The fungal Bromodomain and Extra‐Terminal (BET) protein Bdf1 is a potential antifungal target against invasive fungal infections. One attractive target is the fungal BET protein Bdf1, a global transcriptional regulator. BET proteins bind chromatin through their two bromodomains (BDs), BD1 and BD2, which specifically recognize histones acetylated on lysines. We show that Bdf1 is essential in C. glabrata, and that inactivation of both Bdf1 BDs induces lethality.

Surprisingly, unlike 24 and the other analogs, methylfuryl‐containing compounds 24c and d significantly inhibited CgBD2 in the HTRF assay and inhibited the growth of C. glabrata strains expressing WT Bdf1 and the Bdf1‐Δbd1 mutant. Of the two compounds, 24c exhibited the more potent BD inhibition (IC50 values of 8 and 12 µm against CgBD1 and CgBD2, respectively) and antifungal activity against the WT strain (EC50 value of 90 µM), while displaying only modest cytotoxicity toward HeLa and IMR90 (primary fibroblast) cells at the highest concentration tested (300 µM) in an MTT colorimetric assay. The crystal structure of CgBD1 bound to 24c revealed that the methyltriazine moiety forms direct and water‐mediated H bonds with BC loop residue Asn209 and ZA loop residue Tyr166, respectively. The p‐methylphenyl moiety is recognized by hydrophobic residues Leu161, Ile163, Phe208 and Ile215, including a close contact between the p‐methyl group of 24c and the Ile163 methyl group. Shifting the compound's methyl group to a meta position would abolish this contact and (in one of the two meta positions) yield a steric clash with Phe208, explaining the loss of potency for compounds with this configuration. The methlyfuryl ring packs against Pro151 in the RPF shelf, while the methyl group makes a van der Waals contact with Arg150. Considerable space surrounds this moiety in the binding pocket, explaining why its replacement by certain bulkier substituents is well tolerated. Superimposing the structures of 24 and 24a onto that of 24c reveals that the thiophenyl, furyl and methylfuryl groups of these compounds would all clash with the Tyr327 gauche‐ conformation but that only the methylfuryl group would form a favorable contact with the trans conformation, explaining why compounds 24c and 24d, but not the other analogs, inhibit CgBD2. Namely, whereas CgBD residues Arg150 and Tyr327 point away from the binding pocket, the corresponding Brd4 Trp81 and Typ374 side chains point into the pocket and would clash with the compound's methylfuryl group. In summary, the identification of 24c demonstrates the feasibility of developing inhibitors that target both CgBDs with selectivity over the human BET BDs.

>[4x]GAMGIPQHQQKHALMAIKAVKRLKDARPFLQPVDPVALNIPLYFNFIKRPMDLQTIERKLNANAYETPEQITEDFNLMVENSAKFNGPTAVITQMGRNIQAAFEKHMLNMPAKD>MSSLLNSLLPEYFKPKTNLNINSSRVQYGFNARIDMQYEDDSGTRKGSRPNAFMSNTVAFIGNYEGIIVDDIPILDGLRADIFDTHGDLDMGLVEDALSKSTMIRRNVPTYTAYASELLYKRNLTSLFYNMLRLYYIKKW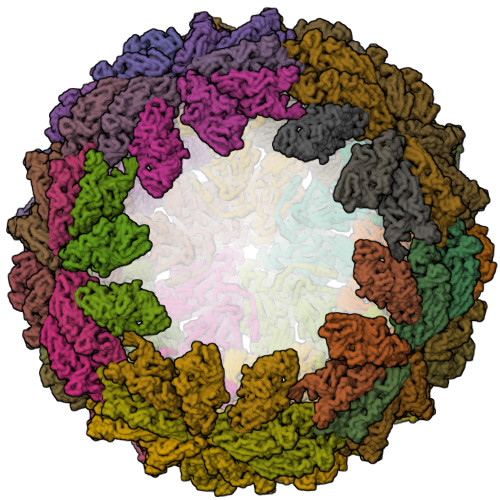GSIKYEKDAIFYDNGHACLLNRQLFPKSRDASLESSLSLPEAEIAMLDPGLEFPEEDVPAILWHGRVSSRATCILGQACSEFAPLAPFSIAHYSPQLTRKLFVNAPAGIEPSSGRYTHEDVKDAITILVSANQAYTDFEAAYLMLAQTLVSPVPRTAEASAWFINAGMVNMPTLSCANGYYPALTNVNPYHRLDTWKDTLNHWVAYPDMLFYHSVAMIESCYVELGNVARVSDSDAINKYTFTELSVQGRPVMNRGIIVDLTLVAMRTGREISLPYPVSCGLTRTDALLQGTEIHVPVVVKDIDMPQYYNAIDKDVIEGQETVIKVKQLPPAMYPIYTYGINTTEFYSDHFEDQVQVEMAPIDNGKAVFNDARKFSKFMSIMRMMGNDVTATDLVTGRKVSNWADNSSGRFLYTDVKYEGQTAFLVDMDTVKARDHCWVSIVDPNGTMNLSYKMTNFRAAMFSRNKPLYMTGGSVRTIATGNYRDAAERLRAMDETLRLKPFKITEKLDFRVAAYAIPSLSGSNMPSLHHQEQLQISEVDAEPINPIGEDELPPDIE[110x]> PQPPKVLSTPLEIAANLRQLQESHDPLIITFHDRSHRFQSYVVHVD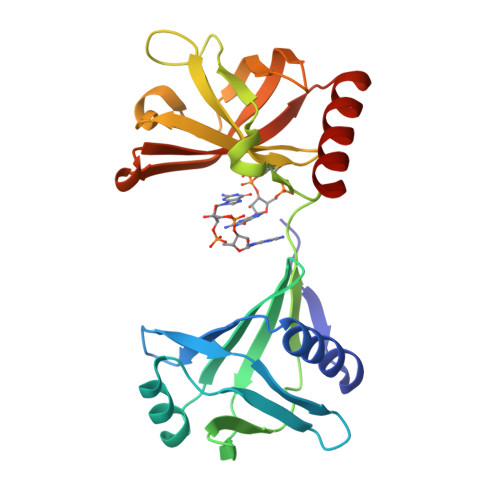RESNTLALDEMIPRDGEKFIENGEHFRVEGFHDGVRIAWECDHALKISEVDGHRCYSGPLPQEVTYHQRRNAFRAALKLSQLVDIILDGAHLKGNGAMRGKLLDISATGCKLRFEGNVEDRLQLGQVYERFKAGNPLGLVDTMVELRHLHYEERINTTFAGVRFHNLSGQAQRKIESFVYQLQRE> GSKLIVDEFEELGEQELDKTTSIYPPETSWEVNKGMNSSRLHKLYSLFFDKSSAFYLGDDVSVLEDKPLTGAYGFQSKKNDQQIFLFRPDSDYVAGYHVDAKSDAGWVNDKLDRRLSEISEFCSKATQPATFILPFVEMPTDITKGVQHQVLLTISYDPKSKQLTPTVYDSIGRDTYSESLSSYFKGKYRTTCDEILTQSIEKAIKSTDFTLGKFT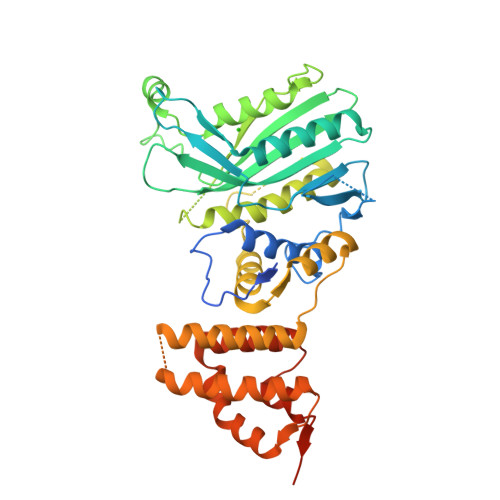RAAYNHQNRLTEGNCGSYTFRTIKEVISSSAQGTEVKIPGSGYITSNSYLTSQHVQDIESCIKYRNLGVVDIESALTEGKTLPVQLSEFIVALEDYGKLRSQQSEKSMLNFIGYSKTAKLTAVELLIGILNDIKGKNEISESQYDKLVKEVDCLMDSSLGKLVQFHLKNLGAESLQKLVLPCVKFDDELFDVPDITGEELASKK>RSPGTLPRKAGVFSDLSNQELKAVHSFLWSKKELRLQPSSTTTMAKNTVFLIEMLLPKKYHVLRFLDKGERHPVREARAVIFFGDQEHPNVTEFAVGPLPGPCYMRALSPRPGYQSSWASRPISTAEYALLYHTLQEATKPLHQFFLNTTGFSFQDCHDRCLAFTDVAPRGVASGQRRSWLIIQRYVEGYFLHPTGLELLVDHGSTDAGH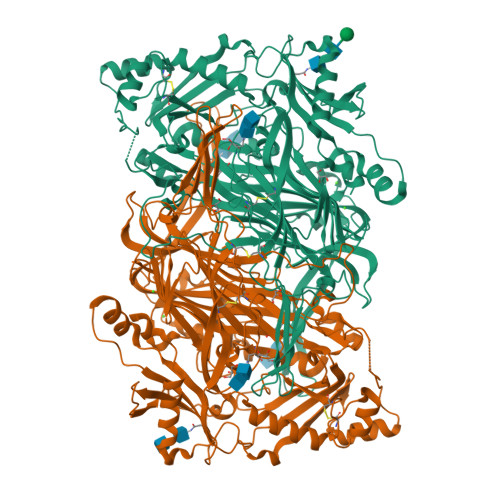WAVEQVWYNGKFYGSPEELARKYADGEVDVVVLEDPLPGGKGHDSTEEPPLFSSHKPRGDFPSPIHVSGPRLVQPHGPRFRLEGNAVLYGGWSFAFRLRSSSGLQVLNVHFGGERIAYEVSVQEAVALYGGHTPAGMQTKYLDVGWGLGSVTHELAPGIDCPETATFLDTFHYYDADDPVHYPRALCLFEMPTGVPLRRHFNSNFKGGFNFYAGLKGQVLVLRTTSTVYNYDYIWDFIFYPNGVMEAKMHATGYVHATFYTPEGLRHGTRLHTHLIGNIHTHLVHYRVDLDVAGTKNSFQTLQMKLENITNPWSPRHRVVQPTLEQTQYSWERQAAFRFKRKLPKYLLFTSPQENPWGHKRSYRLQIHSMADQVLPPGWQEEQAITWARYPLAVTKYRESELCSSSIYHQNDPWDPPVVFEQFLHNNENIENEDLVAWVTVGFLHIPHSEDIPNTATPGNSVGFLLRPFNFFPEDPSLASRDTVIVWPRDNGPNYVQRWIPEDRDCSMPPPFSYNGTYRPV[2x]(2S)-3-(4-amino-3-nitrophenyl)-2-{2-[4-(3,4-dichlorophenyl)-1,3-thiazol-2-yl]hydrazinyl}propanoic 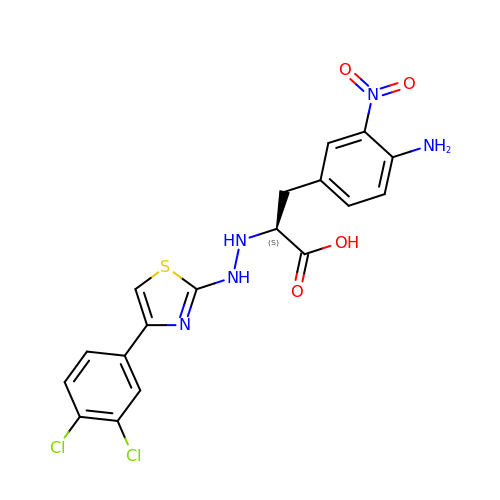acid | C18 H15 Cl2 N5 O4 S | XPSGVIWZSZWGCS-AWEZNQCLSA-N N-ACETYL-P-NITROPHENYLSERINOL | 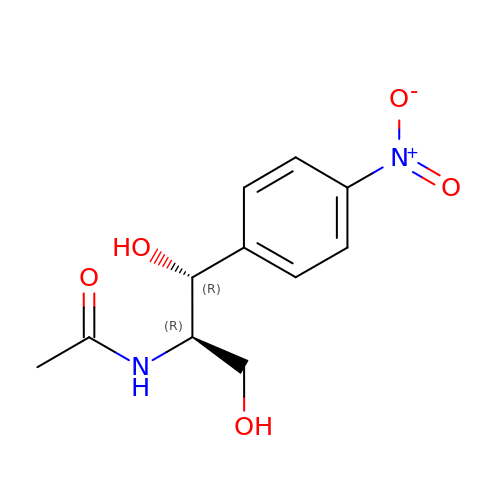C11 H14 N2 O5 | PIVQDUYOEIAFDM-GHMZBOCLSA-N>[4x]MDQKPQPAKTHATEVTVLEGKTMGTFWRASIPGIDAKRSAELKEKIQTQLDADDQLLSTYKKDSALMRFNDSQSLSPWPVSEAMADIVTTSLRIGAKTDGAMDITVGPLVNLWGFGPEQQPVQIPSQEQIDAMK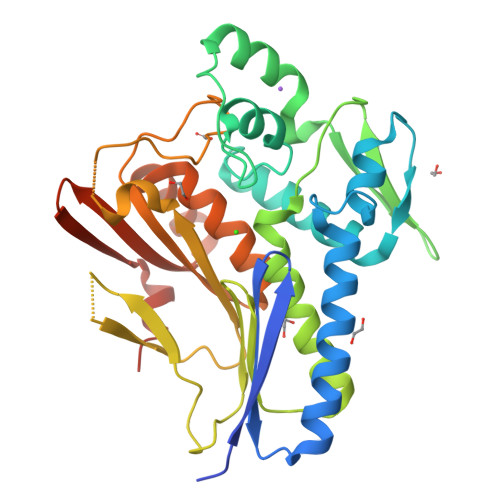AKTGLQHLTVINQSHQQYLQKDLPDLYVDLSTVGEGYAADHLARLMEQEGISRYLVSVGGALNSRGMNGEGLPWRVAIQKPTDKENAVQAVVDINGHGISTSGSYRNYYELDGKRLSHVIDPQTGRPIEHNLVSVTVIAPTALEADAWDTGLMVLGPEKAKEVVRREGLAVYMITKEGDSFKTWMSPQFKSFLVSEKNLEHHHHHH> Y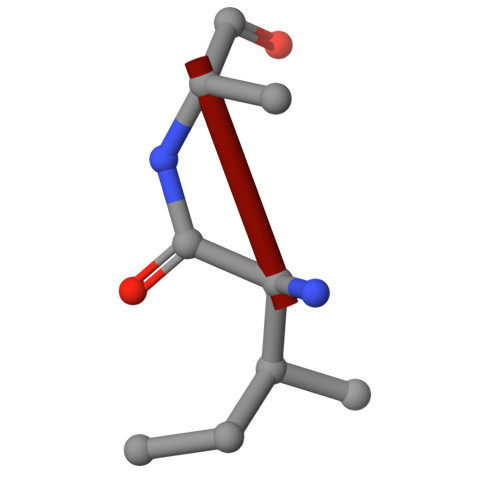PFVEPIK> MQDAITSVINAADVQGRYLDDNSLDKLRGYFQTGELRVRASATIAANAATIIKDSVAKALLYSDITRPGGNMYTTRRYAACIRDLDYYLRYATYGMLAGDPSILDERVL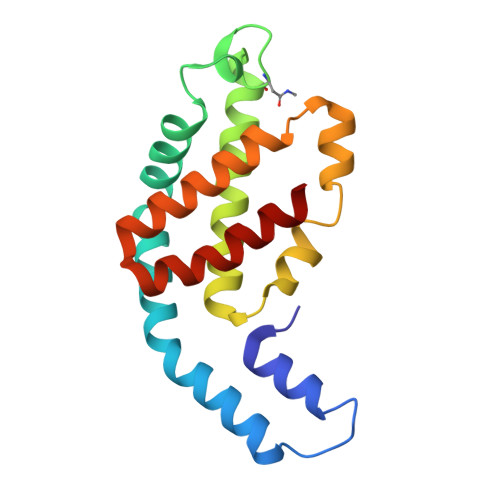NGLKETYNSLGVPIGATIQAVQAMKEVTSSLVGPDAGKEMGVYFDYICSGLS>MKIGVIGAGTMGQGIAKAFAQVEGNTVALCDIKQEWAENGLAKIKKGYEKLVAKGKIPQEKADAIVAAITPGLKENLCADCDLIVEAAFEDMKVKQTTFGELDKICKPECIFASNTSSLSITEIGKGLSRPLVGMHFFNPADRMKLIEVIAGCNTPAETVEKIKEISVAIGKNPVQVNEAAGFVVNRILIPMINEAAFIKMEGVSDIAGIDTAMKLGANHPMGPLELGDFIGLDICLAIMDVLYHETGDSKYRACPLIRKMVRGGNLGCKTGKGFYVYNADRTKTPVDQL[6x]

The A2HBD has elevated expression in F. prausnitzii A2-165 and is crucial for the transformation of acetoacetyl-CoA to 3-hydroxybutyryl-CoA in the butyrate cycle. The monomeric structure of A2HBD consists of two domains, N-terminal and C-terminal, with cofactor binding occurring at the N-terminal domain, while the C-terminal domain facilitates dimerization. The A2HBD protein exists as a hexamer in solution.

The crystal structure of apo-A2HBD was determined at 2.55 Å resolution. The apo form of A2HBD belonged to P21 space group with unit cell parameters a = 87.660 Å, b = 126.611 Å, c = 108.071 Å and α = 90 Å, β = 110.208, γ = 90 Å. The apo-A2HBD protein assembles into an asymmetrical hexameric configuration, wherein all six subunits adopt nearly identical conformations, displaying root-mean-square deviations (RMSD) for the Cα atoms within the range of 0.2 to 0.378 Å. In the asymmetric unit of crystals, it contains three dimers with three two-fold axes.> KETAAAKFERQHMDSSTSAASSSNYCNQMMKSRNLTKDRCKPVNTFVHESLADVQAVCSQKNVACKNGQTNCYQ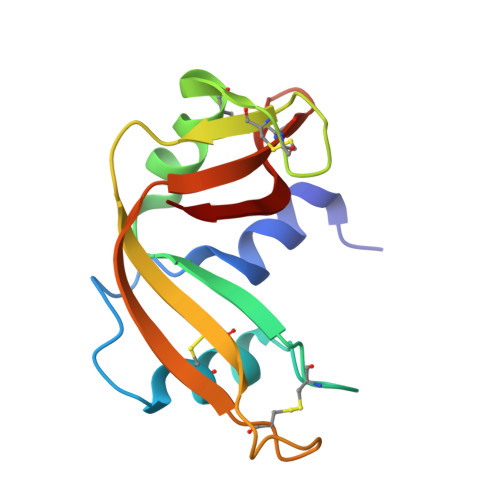SYSTMSITDCRETGSSKYPNCAYKTTQANKHIIVACEGNPYVPVHWDASV> MKITNKSVDKQHIEKLDELRKNVSCTVIGFAEQTAELQQEISELFIAEFGVNGPIDMNSLSKLARITSYYASSEYFQGLAKYQRTACKMFITWQTLRKEAMECRSKDREIFASIPAKLCFFYFYNGELCRAVVCLLDYIDLSDDTLAKEAALRWLMFLGETELIEKKLKTWKMDKSSKDMFSATEFAMNYLKKSEYRVEMLEKLMKLRDKVKSDPTRSFSRYELASYVSWLCSTLSNVPVGSALRECEFPDRVSHIQEAALKSDSLVRNRIPGLASSQFDNSVNASIWPFLDGHQEDSNYYVHIGSTIAWHFEMRRECALVNVTTAQTRDSMSAMILNLRVALKSASFFRVLQTTNTLAYYSSIIEEAGSEK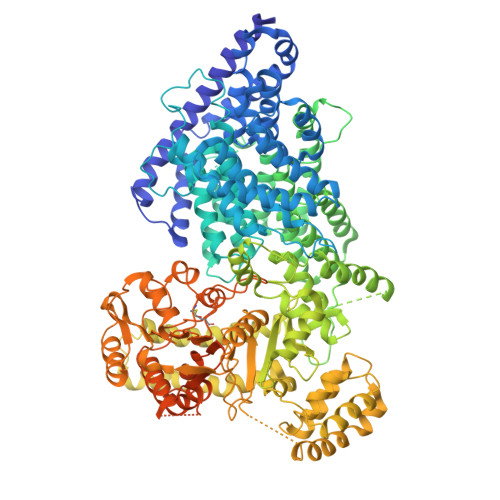NAKLMRVSCVNLLSSNPIIVRCSTPKETGATSRAHTPMAGSSVSEKQNTMRPDLADLLGDLELLDEQSFHPITRSCVCNVCTIYPLHSSFAAEYMMSYAIHSDFSQLSIKHFNDEFARIRERGMSSQVLMHRDSSVRPRPNIIQNEIFGMCVIRWLTKKLDSKESADEDTMEIFNNALKIVRYLQQRTTDMILAVTQLGRQLEFPMECNYSWMRPTIRKPRVKATIDCAVDILRAVSPFGRRPKVEKLEKNLQPFDKERFEKVRLAMRNEMNHYGHILYREWRCRLFAYVGRTSRDPWEAAYAWAESTQIGARNAVQSRLEKCKRGLVTMSGHDRFKTCVQSMPDEMTLVQIAMADDKTIYLVKLHADRDPIIMPLAHYSQAVELMDKFTFLLDEDEMIAKYPGDITPEEFWKRRKIVDGRMMTFVDEVQKHFLGVAASLLMPSGQLGPKAAELAIKIHKLSKGGLLLGEAKEMVYQSKLMDAKSWEALILRFCEMRTTDEKFKSFLPLMHRNSVEVMNQDDSIVTEKKYTYLVICPHLSQFCWERLPIFDEYPYVGRQVSIHSTFSQLEAMKSQEKQIPLQIDVQNAYYILDPDNNLGETQKRMVEYINKFNWEGTVGSAPKSNEISAALSQRDAFFFIGHGSGSSVMPRSVLKQSTCNAISLLMGCGSVRTIPQALGFDGKTAILDYAMAKCPLIVGCLWTVTDGEIDRFLIRMIDDCFEDSKSLTGIDKLRQLSEAMHEARSKARLKYLTGAAVVMYGLPVVAKQTTPFVEKDQRNLPQTPKTSARTSMRMETVPKTPKQEFVTSKSVPMTPIFSNNENKSPSRARMPSRVLKTPRQVKTFQEEDDEAPKRSTTRQLKPLVAPPIPATPTTRTTRSSARTPSRSRNL N~1~,N~1~,N~2~,N~2~-tetramethylhydrazine-1,2-dicarboxamide 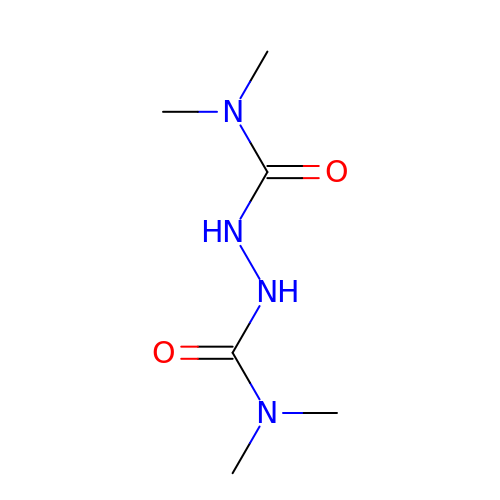| C6 H14 N4 O2 | RAUKYARZDOSMOO-UHFFFAOYSA-N In addition, the molecular interplay of the surface-exposed TlpA (renamed Etrx1) with its extracellular paralogue Etrx2 on oxidative stress resistance and virulence are unknown. This study discovers the unique molecular architecture of two surface-exposed thioredoxin-systems, Etrx1 and Etrx2 and their redox partners CcdA1, CcdA2 and SpMsrAB2 as important pneumococcal extracellular reducing systems essential for pneumococcal pathogenesis and oxidative stress resistance. The bioinformatic analysis of pneumococcal genomes identified two genes encoding surface-exposed thioredoxin-like lipoproteins, renamed here Etrx1 and Etrx2. According to the accepted catalytic mechanism of thioredoxin-like proteins, Etrx1/Etrx2 would bind their redox partner SpMsrAB2 by means of a hydrophobic surface and subsequently perform a nucleophilic attack on the target disulphide bond via the N-terminal nucleophilic thiolate of the CXXC motif (Cys84 in Etrx1, Cys81 in Etrx2). Surface-exposed Etrx1 and Etrx2 deliver electrons to the SpMsrAB2 protein for the reduction of MsrA2 (by Etrx1 or Etrx2) and MsrB2 (by Etrx2) domains.

The three-dimensional structure of Etrx2 in complex with Cyclofos-3™ comprises the sequence from Ile43 to Asn185. Four molecules were found in the asymmetric unit presenting a similar structure (rmsd value of 0.184 Å for all Cα atoms). Etrx2 presents also a modified thioredoxin-like fold that is highly reminiscent of Etrx1 (rmsd value of 1.5 Å for 130 Cα atoms), where the classical thioredoxin-like motif of Etrx2 is embellished by a central αβ insertion and an N-terminal β-hairpin. The CXXC motif (81CGPC84) defines the active site. The main differences between Etrx1 and Etrx2 structures are the presence of eight extra residues forming a coil at the C-terminus of Etrx2, the conformation of β4–α3 loop, the disposition of α3 helix and the more extended conformation of the β7 strand in Etrx2. The Cyclofos-3™ is located in close proximity to the Etrx2 active site. The ligand, found in the four monomers of the asymmetric unit, is stabilized in a pocket formed by the β4–α3 loop, the α4 helix, the α4–β3 loop and the CXXC region. This pocket presents a strong hydrophobic character (Ala78, Trp80, Ala109, Pro110, Ile112, Ala141, Phe144, Ile149, Ile 122) versus the more polar character of the equivalent region in Etrx1. Cyclofos-3™ is stabilized by an H-bond with Gln113, by cation–π interaction of the polar face of the detergent with Trp80 and by pi–pi stacking interaction between phenyl ring of the detergent and Phe144. In the structure of the oxidized forms of Etrx2, a detergent molecule (Cyclofos-3™) or a HED molecule is bound to this hydrophobic pocket, very likely mimicking the redox partner interaction.

>[4x]MKKVMFAGLSLLSLVVLMACGEEETKKTQAAQQPKQQTTVQQIAVGKDAPDFTLQSMDGKEVKLSDFKGKKVYLKFWASWCGPCKKSMPELMELAAKPDRDFEILTVIAPGIQGEKTVEQFPQWFQEQGYKDIPVLYDTKATTFQAYQIRSIPTEYLIDSQGKIGKIQFGAISNADAEAAFKEMN> SRKTYTLTDYLKNTYRLKLYSLRWISDHEYLYKQENNILVFNAEYGNSSVFLENSTFDEFGHSINDYSISPDGQFILLEYNYVKQWRHSYTASYDIYDLNKRQLITEERIPNNTQWVTWSPVGHKLAYVWNNDIYVKIEPNLPSYRITWTGKEDIIYNGITDWVYEEEVF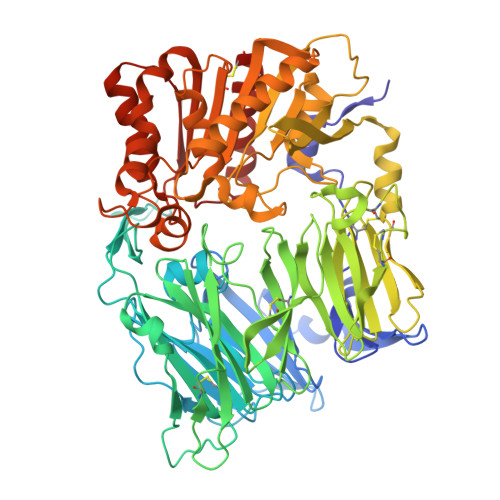SAYSALWWSPNGTFLAYAQFNDTEVPLIEYSFYSDESLQYPKTVRVPYPKAGAVNPTVKFFVVNTDSLSSVTNATSIQITAPASMLIGDHYLCDVTWATQERISLQWLRRIQNYSVMDICDYDESSGRWNCLVARQHIEMSTTGWVGRFRPSEPHFTLDGNSFYKIISNEEGYRHICYFQIDKKDCTFITKGTWEVIGIEALTSDYLYYISNEYKGMPGGRNLYKIQLSDYTKVTCLSCELNPERCQYYSVSFSKEAKYYQLRCSGPGLPLYTLHSSVNDKGLRVLEDNSALDKMLQNVQMPSKKLDFIILNETKFWYQMILPPHFDKSKKYPLLLDVYAGPCSQKADTVFRLNWATYLASTENIIVASFDGRGSGYQGDKIMHAINRRLGTFEVEDQIEAARQFSKMGFVDNKRIAIWGWSYGGYVTSMVLGSGSGVFKCGIAVAPVSRWEYYDSVYTERYMGLPTPEDNLDHYRNSTVMSRAENFKQVEYLLIHGTADDNVHFQQSAQISKALVDVGVDFQAMWYTDEDHGIASSTAHQHIYTHMSHFIKQCFSLP> MELFDENYYAKAVANIIGEVKDPIMYKWFSPDQIEDVDLQMGYQKTVKWDAFLNANPTTIANEVNTISTIGFSSEVVRLNYLKLQYKFRHLKQTSEKFYTSDSYIGDINNNLLPFAQAYKLASSEIIKLINHFVLTGTVSIQKDGKNQKRLLPNMYGLLNMPEQIKEEVASGDKDKMDKIFEKIEAGLSKLELGDEFSTPMMVIVDPATSLKLVKPYAAAQGAASSCEKWEDVLIQTIKAINNREDVYIETSNLLKHKILIYPLNSELIKFKPSKYMLPTPNEQVDKD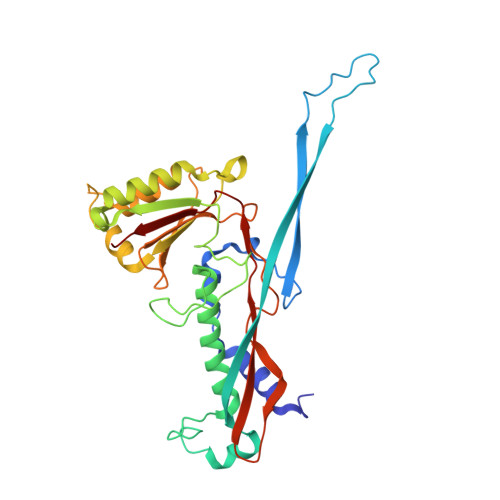STDVAHSYIDFVLGGLLATRKTILQVNIKQS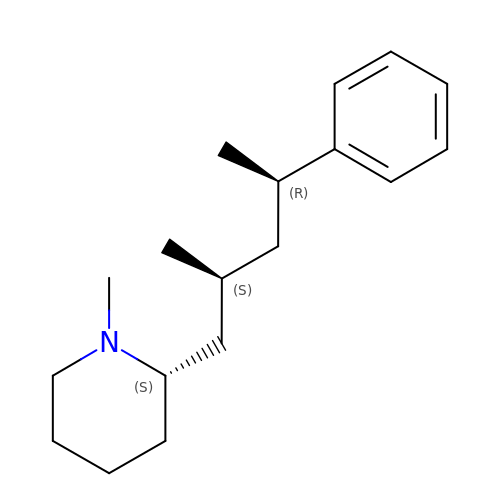(2S)-1-methyl-2-[(2S,4R)-2-methyl-4-phenylpentyl]piperidine | C18 H29 N | UEEAJOUBQAEABH-JZXOWHBKSA-N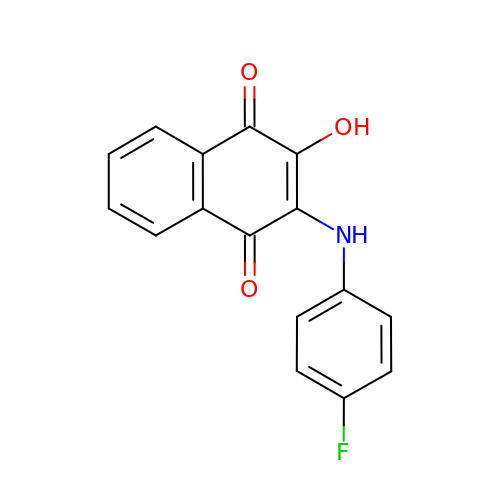2-[(4-fluorophenyl)amino]-3-hydroxynaphthalene-1,4-dione | C16 H10 F N O3 | AVGHWZUEYVXFON-UHFFFAOYSA-N> KHLPEPFRIRVIEPVKRTTRAYREEAIIKSGMNPFLLDSEDVFIDLLTDSGTGAVTQSMQAAMMRGDEAYSGSRSYYALAESVKNIFGYQYTIPTHQGRGAEQIYIPVLIKKREQEKGLDRSKMVAFSNYFFDTTQGHSQINGCTVRNVYIKEAFDTGVRYDFKGNFDLEGLERGIEEVGPNNVPYIVATITSNSAGGQPVSLANLKAMYSIAKKYDIPVVMDSARFAENAYFIKQREAEYKDWTIEQITRETYKYADMLAMSAKKDAMVPMGGLLCMKDDSFFDVYTECRTLCVVQEGFPTYGGLEGGAMERLAVGLYDGMNLDWLAYRIAQVQYLVDGLEEIGVVCQQAGG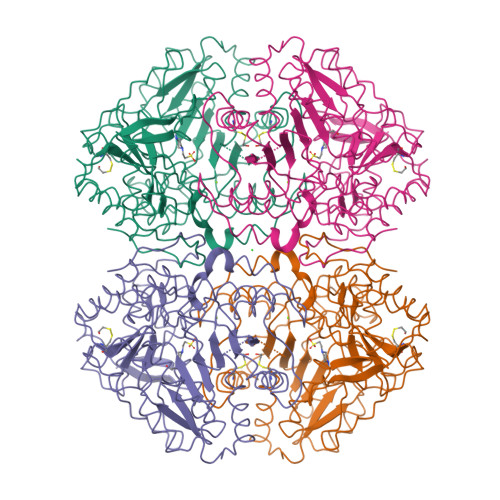HAAFVDAGKLLPHIPADQFPAQALACELYKVAGIRAVEIGSFLLGRDPKTGKQLPCPAELLRLTIPRATYTQTHMDFIIEAFKHVKENAANIKGLTFTYEPKVLRHFTAKLKEV>MYTNSDFVVIKALEDGVNVIGLTRGADTRFHHSEKLDKGEVLIAQFTEHTSAIKVRGKAYIQTRHGVIESEGK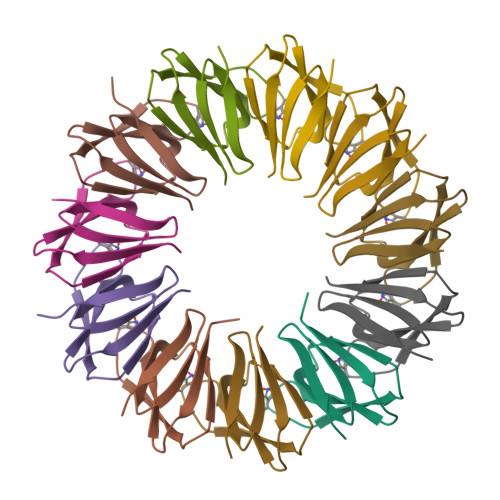K[22x]>AEVTQLSNGIVVATEHNPSAHTASVGVVFGSGAANENPYNNGVSNLWKNIFLSKENSAVAAKEGLALSSNISRDFQSYIVSSLPGSTDKSLDFLNQSFIQQKANLLSSSNFEATKKSVLKQVQDFEENDHPNRVLEHLHSTAFQNTPLSLPTRGTLESLENLVVADLESFANNHFLNSNAVVVGTGNIKHEDLVNSIESKNLSLQTGTKPVLKKKAAFLGSEVRLRDDTLPKAWISLAVEGEPVNSPNYFVAKLAAQIFGSYNAFEPASRLQGIKLLDNIQEYQLCDNFNHFSLSYKDSGLWGFSTATRNVTMIDDLIHFTLKQWNRLTISVTDTEVERAKSLLKLQLGQLYESGNPVNDANLLGAEVLIKGSKLSLGEAFKKIDAITVKDVKAWAGKRLWDQDIAIAGTGQIEGLLDYMRIRSDMSMMRW[2x];>LTVSARDAPTKISTLAVKVHGGSRYATKDGVAHLLNRFNFQNTNTRSALKLVRESELLGGTFKSTLDREYITLKATFLKDDLPYYVNALADVLYKTAFKPHELTESVLPAARYDYAVAEQCPVKSAEDQLYAITFRKGLGNPLLYDGVERVSLQDIKDFADKVYTKENLEVSGENVVEADLKRFVDESLLSTLPAGKSLVSKSEPKFFLGEENRVRFIGDSVAAIGIPVNKASLAQYEVLANYLTSALSELSGLISSAKLDKFTDGGLFTLFVRDQDSAVVSSNIKKIVADLKKGKDLSPAINYTKLKNAVQNESVSSPIELNFDAVKDFKLGKFNYVAVGDVSNLPYLDEL[2x];>[2x]MAFRKSNVYLSLVNSYIIDSPQPSSINYWWNMGSLLGLCLVIQIVTGIFMAMHYSSNIELAFSSVEHIMRDVHNGYILRYLHANGASFFFMVMFMHMAKGLYYGSYRSPRVTLWNVGVIIFILTIATAFLGYCCVYGQMSHWGATVITNLFSAIPFVGNDIVSWLWGGFSVSNPTIQRFFALHYLVPFIIAAMVIMHLMALHIHGSSNPLGITGNLDRIPMHSYFIFKDLVTVFLFMLILALFVFYSPNTLGHPDNYIPGNPLVTPASIVPEWYLLPFYAILRSIPDKLLGVITMFAAILVLLVLPFTDRSVVRGNTFKVLSKFFFFIFVFNFVLLGQIGACHVEVPYVLMGQIATFIYFAYFLIIVPVISTIENVLFYIGRVNK;>[2x]MTAAEHGLHAPAYAWSHNGPFETFDHASIRRGYQVYREVCAACHSLDRVAWRTLVGVSHTNEEVRNMAEEFEYDDEPDEQGNPKKRPGKLSDYIPGPYPNEQAARAANQGALPPDLSLIVKARHGGCDYIFSLLTGYPDEPPAGVALPPGSNYNPYFPGGSIAMARVLFDDMVEYEDGTPATTSQMAKDVTTFLNWCAEPEHDERKRLGLKTVIILSSLYLLSIWVKKFKWAGIKTRKFVFNPPKPRK;>KSTYRTPNFDDVLKENNDADKGRSYAYFMVGAMGLLSSAGAKSTVETFISSMTATADVLAMAKVEVNLAAIPLGKNVVVKWQGKPVFIRHRTPHEIQEANSVDMSALKDPQTDADRVKDPQWLIMLGICTHLGCVPIGEAGDFGGWFCPCHGSHYDISGRIRKGPAPLNLEIPAYEFDGDKVIVG[2x];> VTDQLEDLREHFKNTEEGKALVHHYEECAERVKIQQQQPGYADLEHKEDCVEEFFHLQHYLDTATAPRLFDKLK;>PQSFTSIARIGDYILKSPVLSKLCVPVANQFINLAGYKKLGLKFDDLIAEENPIMQTALRRLPEDESYARAYRIIRAHQTELTHHLLPRNEWIKAQEDVPYLLPYILEAEAAAKEKDELDNIEVSK[2x];>[2x]GPPSGKTYMGWWGHMGGPKQKGITSYAVSPYAQKPLQGIFHNAVFNSFRRFKSQFLYVLIPAGIYWYWWKNGNEYNEFLYSKAGREELERVNV;> SLYKTFFKRNAVFVGTIFAGAFVFQTVFDTAITSWYENHNKGKLWKDVKARIAA;> EVTDQLEDLREHFKNTEEGKALVHHYEECAERVKIQQQQPGYADLEHKEDCVEEFFHLQHYLDTATAPRLFDKLK;> SSLYKTFFKRNAVFVGTIFAGAFVFQTVFDTAITSWYENHNKGKLWKDVKARIA;> KTGLHFGRLSLRSLTAYAPNLMLWGGASMLGLFVFTEGWPKFQD;> TGLHFGRLSLRSLTAYAPNLMLWGGASMLGLFVFTEGWPKFQDTLYKKIPL;> WLYSTNAKDIAVLYFMLAIFSGMAGTAMSLIIRLELAAPGSQYLHGNSQLFNVLVVGHAVLMIFFLVMPALIGGFGNYLLPLMIGATDTAFPRINNIAFWVLPMGLVCLVTSTLVESGAGTGWTVYPPLSSIQAHSGPSVDLAIFALHLTSISSLLGAINFIVTTLNMRTNGMTMHKLPLFVWSIFITAFLLLLSLPVLSAGITMLLLDRNFNTSFFEVSGGGDPILYEHLFWFFGHPEVYILIIPGFGIISHVVSTYSKKPVFGEISMVYAMASIGLLGFLVWSHHMYIVGLDADTRAYFTSATMIIAIPTGIKIFSWLATIHGGSIRLATPMLYAIAFLFLFTMGGLTGVALANASLDVAFHDTYYVVGHFHYVLSMGAIFSLFAGYYYWSPQILGLNYNEKLAQIQFWLIFIGANVIFFPMHFLGINGMPRRIPDYPDAFAGWNYVASIGSFIATLSLFLFIYILYDQLVNGLNNKVNNKSVIYNKAPDFVESNTIFNLNTVKSSSIEFLLTSPPAVHSFNTPAVQS;> DVPTPYACYFQDSATPNQEGILELHDNIMFYLLVILGLVSWMLYTIVMTYSKNPIAYKYIKHGQTIEVIWTIFPAVILLIIAFPSFILLYLCDEVISPAMTIKAIGYQWYWKYEYSDFINDSGETVEFESYVIPDELLEEGQLRLLDTDTSMVVPVDTHIRFVVTAADVIHDFAIPSLGIKVDATPGRLNQVSALIQREGVFYGACSELCGTGHANMPIKIEAVSLPKFLEWLNEQ;> THLERSRHQQHPFHMVMPSPWPIVVSFALLSLALSTALTMHGYIGNMNMVYLALFVLLTSSILWFRDIVAEATYLGDHTMAVRKGINLGFLMFVLSEVLIFAGLFWAYFHSAMSPDVTLGACWPPVGIEAVQPTELPLLNTIILLSSGATVTYSHHALIAGNRNKALSGLLITFWLIVIFVTCQYIEYTNAAFTISDGVYGSVFYAGTGLHFLHMVMLAAMLGVNYWRMRNYHLTAGHHVGYETTIIYTHVLDVIWLFLYVVFYWWGV;> VVKTAQNLAEVNGPETLIGPGAKEGTVPTDLDQETGLARLELLGKLEGIDVFDTKPLDSSRKGTMKDPIIIESYDDYRYVGCTGSPAGSHTIMWLKPTVNEVARCWECGSVYKLNPV;> ALSNAAVMDLQSRWENMPSTEQQDIVSKLSERQKLPWAQLTEPEKQAVWYISYGEWGPRRPVLNKGDSSFIAKGVAAGLLFSVGLFAVVRMAGGQDAKTMNKEWQLKSDEYLKSKNANPWGGYSQVQS;> ETFEEFTARYEKEFDEAYDLFEVQRVLNNCFSYDLVPAPAVIEKALRAARRVNDLPTAIRVFEALKYKVENEDQYKAYLDELKDVRQELGVPLKEELFP;> NKVIQLQKIFQSSTKPLWWRHPRSALYLYPFYAIFAVAVVTPLLYIPNAIRGIKA;> VHFKDGVYENIPFKVKGRKTPYALSHFGFFAIGFAVPFVACYVQLKKSGAF;> IAPITGTIKRRVIMDIVLGFSLGGVMASYWWWGFHMDKINKREKFYAELAERK;> NSPLHTVGFDARFPQQNQTKHCWQSYVDYHKCVNMKGEDFAPCKVFWKTYNALCPLDWIEKWDDQREKGIFAGDINSD;> NALKPAFGPPDKVAAQKFKESLMATEKHAKDTSNMWVKISVWVALPAIALTAVNTYFVEKEHAEHREHLKHVPDSEWPRDYEFMNIRSKPFFWGDGDKTLFWNPVVNRHIEHDD;> ESWVITEGRRLIPEIFQWSAVLSVCLGWPGAVYFFSKA

Respiratory chains are crucial for cellular energy conversion and consist of multi‐subunit complexes that can assemble into supercomplexes. In mammalian cells, the mitochondrial respiratory chain (MRC) is formed by four distinct complexes (CI–CIV) (Lobo‐Jarne & Ugalde, 2018). Together with the ATP synthase (CV), these complexes form the oxidative phosphorylation (OXPHOS) system, in which electron transfer to molecular oxygen is coupled with the formation of an electrochemical gradient over the inner mitochondrial membrane to drive ATP synthesis. Three major models have been proposed for the structural organization of the MRC: the solid‐state, the liquid‐state (fluid), and the plasticity model (Acín‐Pérez et al, 2008; Milenkovic et al, 2017; Lobo‐Jarne & Ugalde, 2018). The latter consolidates the previous two models and is based on findings from the past two decades, showing that MRC complexes are not randomly distributed within the inner mitochondrial membrane, but can be assembled into supramolecular structures termed supercomplexes (SCs). In summary, our results demonstrate that the formation of SCs is important for efficient electron transfer between CIII and CIV by positioning the Cyt c binding sites of both complexes in close vicinity, a conserved feature of SC architecture found in multiple organisms.

Particles from a dataset previously acquired (Rathore et al, 2019) were re‐processed using an updated version of the software cryoSPARC (Punjani et al, 2017) (Fig EV1A; Table EV1). Non‐uniform refinement of these particles generated a 3.17 Å density map (GSFSC = 0.143; B‐factor: −107.1; Fig EV1B), which was used to model the CIII2/CIV respiratory SC. The 3.17 Å (FSC = 0.143) density map of the CIII2/CIV SC was used for model building the SC in Coot v0.8.8 (Emsley et al, 2010). A Side view of the overall structure of the Saccharomyces cerevisiae CIII2/CIV supercomplex and its position in the mitochondrial inner membrane (IM). The improved resolution of the matrix‐localized protein–protein interactions between the CIII‐subunit Cor1 and the CIV protein Cox5a also enabled unequivocal identification of the residues connecting the two complexes. In addition to the Cor1‐Cox5a protein–protein interaction, CIII and CIV also interact with each other through a CL molecule situated between Cox5a and Rip1. Moreover, we could confirm that the protein–lipid–protein interactions between Cox5a and Rip1 contained cardiolipin (CL), as previously suggested (Hartley et al, 2019). The inner membrane protein–lipid–protein interactions (Rip1‐CL-Cox5a), where Rip1 is marked in gold, cardiolipin (CL) in gray, and Cox5a in red (B), and the mitochondrial matrix, protein–protein interaction of Cor1 (blue), and Cox5a (red) (C) are shown. However, the absence of CL per se did not abolish SC formation in our experimental setup, revealing that the Cor1–Cox5a interaction is necessary and sufficient for forming SCs.>[2x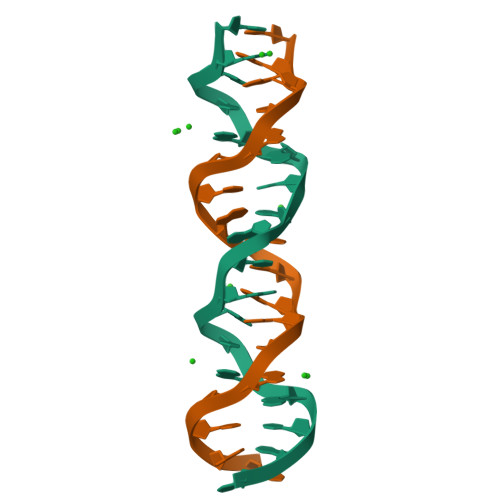]CGACGACGACGACGATGA>MALNSINTNSGALIALQNLNSTNAELTQVQQRINTGKKIGSAKDNGAIWATAKNQSATAGSMNAVKDSLQRGQSTIDVALAAGDTITDLLGKMKEKALAASDTS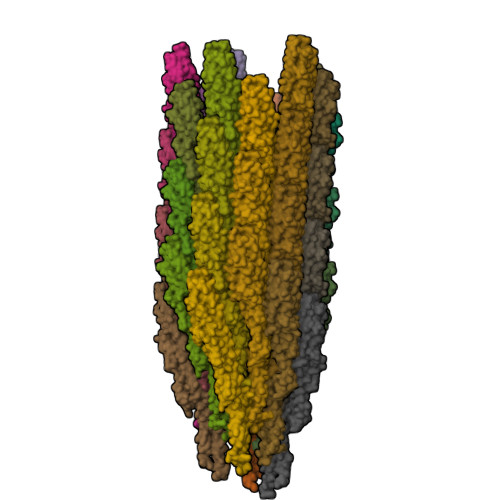LNTASFNALKSDFDSLRDQITKAASNAKFNGVSIADGTTTKLSFLANSDGSAFTVTAKTLTLGGLGLTATSSFTTAAAAKTMIGTIDTALQTATNKLASLGTSSTGLDTHLTFVGKLQDSLDAGVGNLVDADLAKESAKLQSLQTKQQLGVQALSIANQSSSSILSLFR[38x]>SNAMLIKPKRLQPGDIVATVSPSWGGAGDSEIRWRYEQGVKRLEEVFGLTVVPMPNSLKGSEFIYNNPQARAEDLMTAFQDTRVKAIIANIGGQDSIRLLPYIDFNAIRENPKIFMGYADVTISHLFCHKAGLSSFYGPAILTDFAENVEMDPYTVEMVNRTLFSNEMIGEIQPAPEWTSERLEWIEINKDTRRTMQQNNGYELLQGSTTVQGRLIGGCIEVLEFAKGTELWPEKKHWEDSILFFATSEDHPEPSYIKYWLRNYAAQGI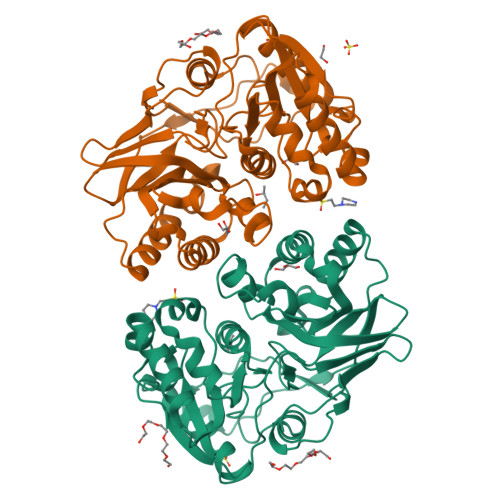LQKAKGIIFGKPKDEMYYEEYKHEILQVMKEHNLEDLPILYNLNFGATEPKFILPYGSMAEIDCENGSFSILESGVE[2x]(3R)-4-(4-chlorophenyl)-1-[(3S,4R)-3-(4-chlorophenyl)-4-(hydroxymethyl)pyrrolidin-1-yl]-3-hydroxybutan-1-one | C21 H23 Cl2 N O3 | 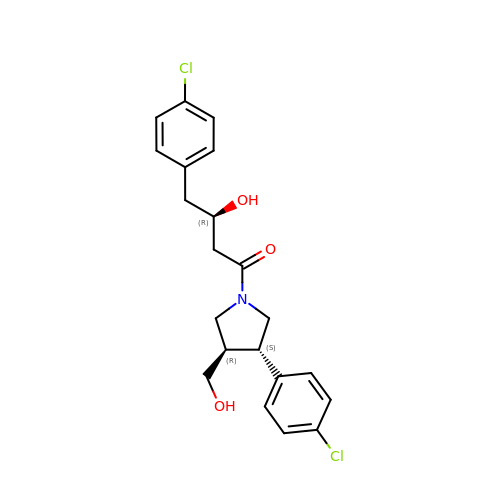PKCGAGXONWDTRK-NSISKUIASA-N> MGSSHHHHHHENLYFQGCDWQRTSKERSKNAQNQQVIKIGYLPITHSANLMMTKKLLSQYNHPKYKLELVKFNNWPDLMDALNSGRIDGASTLI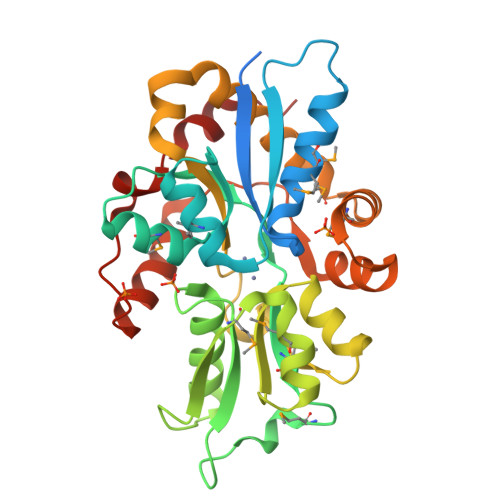ELAMKSKQKGSNIKAVALGHHEGNVIMGQKGMHLNEFNNNGDDYHFGIPHRYSTHYLLLEELRKQLKIKPGHFSYHEMSPAEMPAALSEHRITGYSVAEPFGALGEKLGKGKTLKHGDDVIPDAYCCVLVLRGELLDQHKDVAQAFVQDYKKSGFKMNDRKQSVDIMTHHFKQSRDVLTQSAAWTSYGDLTIKPSGYQEITTLVKQHHLFNPPAYDDFVEPSLYKEASRS>FACKTANGTAIPIGGGSANVYVNLAPVVNVGQNLVVDLSTQIFCHNDYPETITDYVTLQRGSAYGGVLSNFSGTVKYSGSSYPFPTTSETPRVVYNSRTDKPWPVALYLTPVSSAGGVAIKAGSLIAVLILRQTNNYNSDDFQFVWNIYANNDVVVPTGGCDVSARDVTVTLPDYPGSVPIPLTVYCAKSQNLGYYLSGTTADAGNSIFTNTASFSPAQGVGVQLTRNGTIIPANNTVSLGAVGTSAVSLGLTANYARTGGQVTAGNVQSIIGVTFVYQ[4x];>ADSTITIRGYVRDNG[4x]

The adhesin FimH at the fimbrial tip specifically binds in a catch-bond mode to terminal α-D-linked mannoses of N-linked glycans of the receptor uroplakin 1a on urinary epithelial cells. FimH is a two-domain protein, composed of an N-terminal, mannoside-binding lectin domain (FimHL) and a C-terminal pilin domain (FimHP). FimHP possesses an incomplete immunoglobulin-like fold that is completed by insertion of an N-terminal donor strand of FimG, the subsequent subunit in pilus assembly. The two-domain architecture of FimH is a prerequisite for catch-bond formation because the interactions between FimHL and FimHP determine the conformational state and ligand-binding properties of FimHL.

We had shown previously that FimHP also accepts the donor strand of the non-cognate subunit FimF (DsF). However, FimHP is slightly less stabilized by complementation with DsF than with the natural donor-strand DsG30. We hypothesized that such complementation with DsF instead of DsG could also result in a mild destabilization of the interdomain interface in full-length FimH. We then determined the co-crystal structure of FimHK12·DsF with HM (FimHK12·DsF·HM) at 3.0 Å resolution with four molecules in the asymmetric unit. Three FimHK12·DsF·HM molecules closely resembled the Abound state (r.m.s.d. of 0.6 Å to FimHF18·DsG·HM) with a preserved interdomain interface. In the fourth molecule, however, the FimHL and FimHP domains were separated and they adopted a drastically different relative orientation with an angle between the domains of ∼45° instead of ∼150° in the other three molecules. Remarkably, in the bent fourth molecule, no interactions between FimHL and FimHP other than the direct covalent linkage are detected, equivalent to a breakdown of the total 500 Å2 interdomain interface of the Abound state. This molecule thus represents a third state, the domain-Separated, ligand-bound state of FimH, Sbound. The complete absence of non-covalent interdomain interactions indicates that the Sbound state does not possess a defined relative domain orientation in solution, and that the observed, kinked conformation has been selected only by crystal packing. In this Sbound state, FimHL adopts a conformation closely resembling isolated FimHL with bound ligand.>[2x]MCPSACKCTVSLYGEMVVACGGMGLTEIPEDIPHRAVYLVLKDNNITKITSYSFKGLRNLQGIDLSNNKINHISSAALRHLGHLDDIDLSRNELTSVSEKLFDFPISSAKAQGRRFFVYLANNPWGCDCRMAWLAQELAGGSKTFGDRHMECATPAALAGRGLSEIPQTSFVCTGRDISFDSD

VLRs are featured with a LRR domain of multiple LRR modules and an invariant stalk region rich in threonine and proline residues2. Jawless vertebrate AIS employs VLRs as antigen receptors to recognize invaded pathogens, such as viruses and bacteria. In summary, we identified Bf66946 from B. floridae as an analog of variable lymphocyte receptor VLRC using bioinformatics analysis and structural comparison combined with in vitro bacterial binding assays. This is the first characterized VLR-like protein in amphioxus, suggesting the emergence of VLR-based AIS in basal chordates.

We applied both the recombinant Bf66946 and Bf289081 to crystallization trials; however, only the crystal structure of Bf66946 was successfully determined at a resolution of 1.79 Å in the space group P212121. Each asymmetric unit contains two molecules with a total buried interface area of 567 Å2, which is not sufficient to maintain a stable dimer. In fact, gel-filtration chromatography also indicated that Bf66946 exists as a monomer in solution. The overall structure of Bf66946 (residues Cys21–Asp202) adopts a crescent-shaped solenoid conformation, rich of conserved leucine and isoleucine residues involved in formation of the hydrophobic core, which is typical for the LRR family. The structure contains a 36-residue LRRNT, an 18-residue LRR1, two 24-residue LRRVs (LRRV1 and LRRVe), a 20-residue CP and a 51-residue LRRCT. The inner concave surface of Bf66946 is formed by a β-sheet made up of six β-strands (β1, β2, β3, β5, β7 and β8), with β1 anti-parallel to the remaining β-strands that are arranged in a parallel fashion. Notably, the 20-residue CP in Bf66946 folds into an α-helix that shares no identity with the 13-residue CP of previously identified VLRs. Moreover, the N- and C-terminal caps of Bf66946 also have four strictly conserved disulfide bonds presumably important for the structural integrity: two within LRRNT (Cys21-Cys27, Cys25-Cys39) and the other two within LRRCT (Cys146-Cys171, Cys148-Cys192). Altogether, lamprey VLRA and VLRB possess an insertion in LRRCT, whereas Bf66946 and lamprey VLRC possess a protruding loop in LRRNT, suggesting that Bf66946 is more likely a putative VLRC rather than either VLRA or VLRB. Thus, we identified that the residues Asp105 and Asp107 at the concave are key to recognition of Gram-positive bacteria.>SNAMKLTPNYYRDRVCLNVLAGSKDNARAIYQAAEGHVLVGVLSKNYPDVDSAVKDMREYAALIDNALSVGLGAGDPRQSVMVSQISQQVQPQHVNQVFTGVGASRALLGQHDTVVNGLISPTGKVGYVKISTGPLSSQQKDAIVPVTTAIAMLKDMGGSSVKFFPMNGLDSIDEYRFVAEACAATGFWLEPTGGIDLDNFEQIVQIALDAGVTKVIPHIYSSIIDSK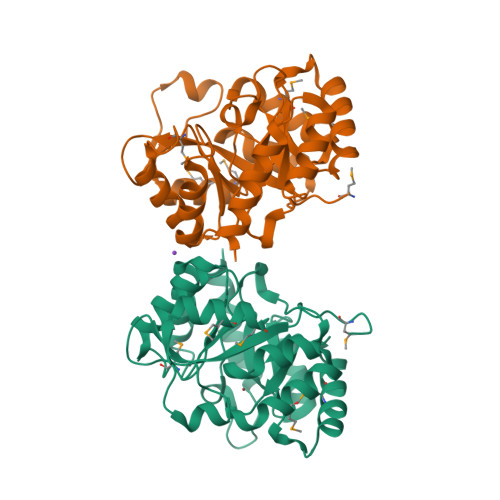TGNTRPEDVKTLLDIVKKIVQ[2x]>[2x]MLTYQVKQGDTLNSIAADFRISTAALLQANPSLQAGLTAGQSIVIPGLPDPYTIPYHIAVSIGAKTLTLSLNNRVMKT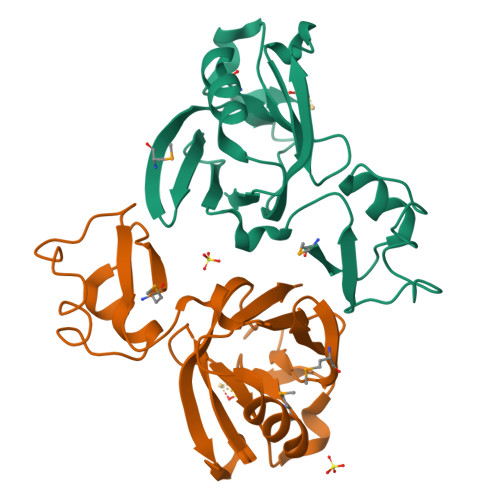YPIAVGKILTQTPTGEFYIINRQRNPGGPFGAYWLSLSAAHYGIHGTNNPASIGKAVSKGCIRMHNKDVIELASIVPNGTRVTINR> MPLDPVIQQVLDQLNRMPAPDYKHLSAQQFRSQQSLFPPVKKEPVAEVREFDMDLPGRTLKVRMYRPEGVEPPYPALVYYHGGGWVVGDLETHDPVCRVLAKDGRAVVFSVDYRLAPEHKFPAAVEDAYDALQWIAERAADFHLDPARIAVGGDSAGGNLAAVTSILAKERGGPAIAFQLLIYPSTGYDPAHPPASIE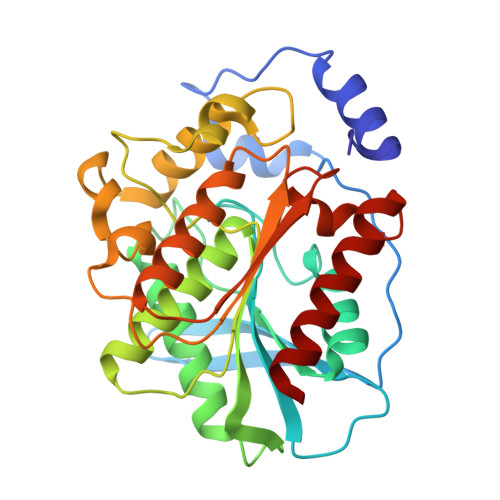ENAEGYLLTGGMMLWFRDQYLNSLEELTHPWFSPVLYPDLSGLPPAYIATAQYDPLRDVGKLYAEALNKAGVKVEIENFEDLIHGFAQFYSLSPGATKALVRIAEKLRDALA>GSDYIIKEKTVLLQKKDSEGFGFVLRGAKAQ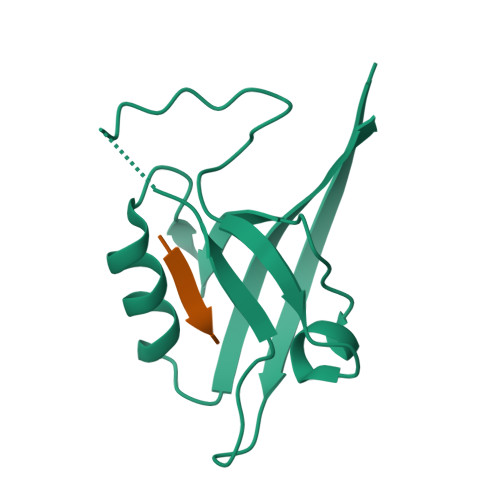TPIEEFTPTPAFPALQYLESVDEGGVAWRAGLRMGDFLIEVNGQNVVKVGHRQVVNMIRQGGNTLMVKVVMVTRHPDMDEAVHK[8x];>[8x]AWDETNL N-[3-(4-{[(2-aminoethyl)(methyl)amino]methyl}-1H-pyrrol-3-yl)phenyl]prop-2-enamide 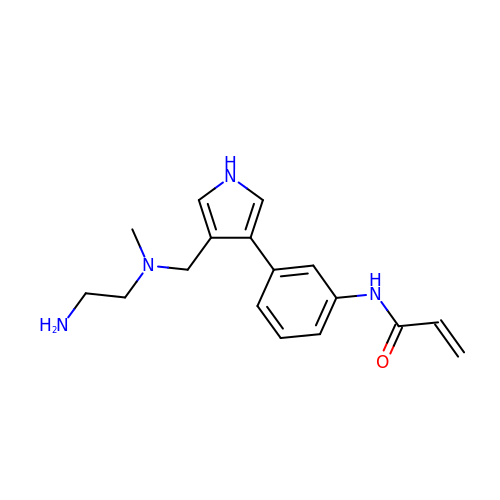| C17 H22 N4 O | HVDMIAFOVVMNJF-UHFFFAOYSA-N>[2x]MCELLGMSANVPTDIVFSFTGLMQRGGGTGPHRDGWGIAFYEGRGVRLFQDPLASVDSEVARLVQRFPIKSETVIGHIRQANVGKVGLSNTHPFIRELGGRYWTFAHNGQLADFQPKPGFYRPVGETDSEAAFCDLLNRVRRAFPEPVPVEVLLPVLISACDEYRKKGVFNALISDGDWLFTFCSSKLA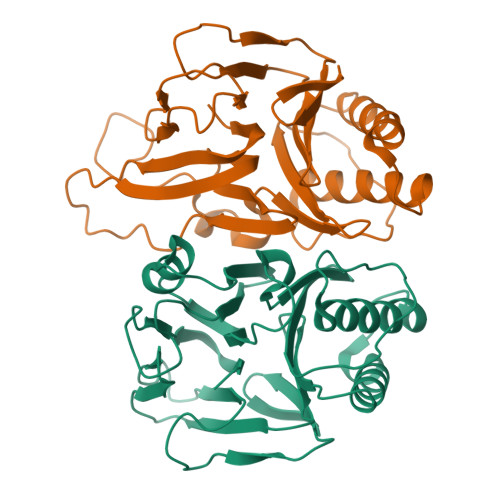YITRRAPFGPARLKDADLTVDFHAETTPDDVVTVIATEPLTDNENWTLQQSGEWVLWWGGEVLAKGRV> MTVRKNQATLTADEKRRFVAAVLELKRSGRYDEFVRTHNEFIMSDTDSGERTGHRSPSFLPWHRRFLLDFEQALQSVDSSVTLPYWDWSADRTVRASLWAPDFLGGTGRSTDGRVMDGPFAASTGNWPINVRVDSRTYLRRSLGGSVAELPTRAEVESVLAISAYDLPPYNSASEGFRNHL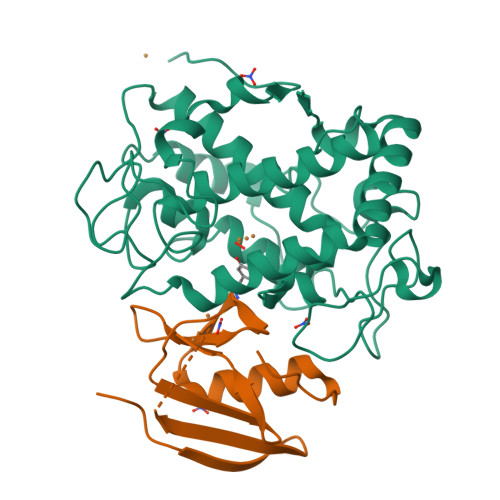EGWRGVNLHGRVHVWVGGQMATGVSPNDPVFWLHHAYVDKLWAEWQRRHPDSAYVPTGGTPDVVDLNETMKPWNTVRPADLLDHTAYYTFDALEHHHHHH;> MPEITRRRALTAAAAVAATASAAVTLAAPAASAAGHHEPAAPESFDEVYKGRRIQGRPARGAAHHHEHGGGYEVFVDGVQLHVMRNADGSWISVVSHYDPVPTPRAAARAAVDELQGAPLLPFPANLEHHHHHH>MKIGSGEKLLFIGDSITDCGRARPEGEGSFGALGTGYVAYVVGLLQAVYPELGIRV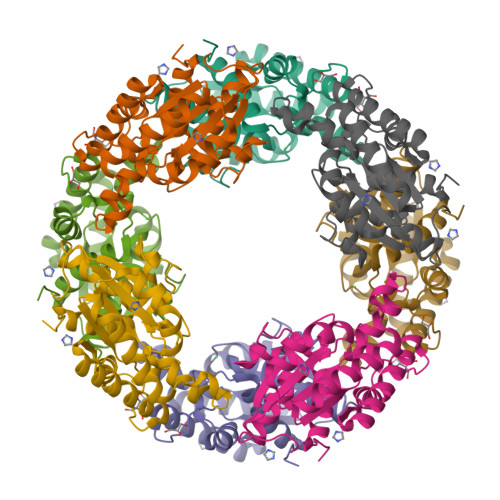VNKGISGNTVRDLKARWEEDVIAQKPDWVSIMIGINDVWRQYDLPFMKEKHVYLDEYEATLRSLVLETKPLVKGIILMTPFYIEGNEQDPMRRTMDQYGRVVKQIAEETNSLFVDTQAAFNEVLKTLYPAALAWDRVHPSVAGHMILARAFLREIGFEIVRSR[2x]>[2x]MNDALHIGLPPFLVQANNEPRVLAAPEARMGYVLELVRANIAADG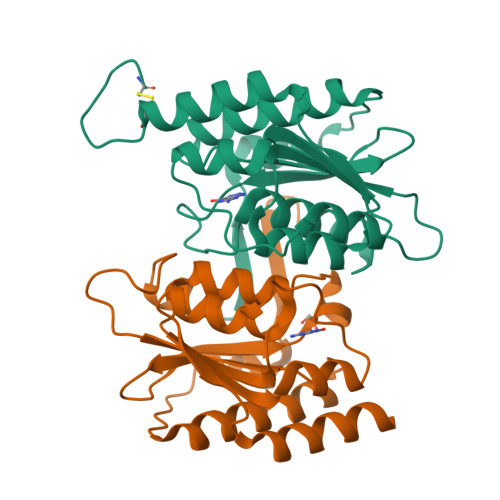GPFAAAVFERDSGLLIAAGTARVVPGRCSAAHAEILALSLAQAKLDTHDLSADGLPACELVTSAEPCVMCFGAVIWSGVRSLVCAARSDDVEAIGFDEGPRPENWMGGLEARGITVTTGLLRDAACALLREYNACNGVIYNARCGVHK> MGSSHHHHHHSQDPMEIDE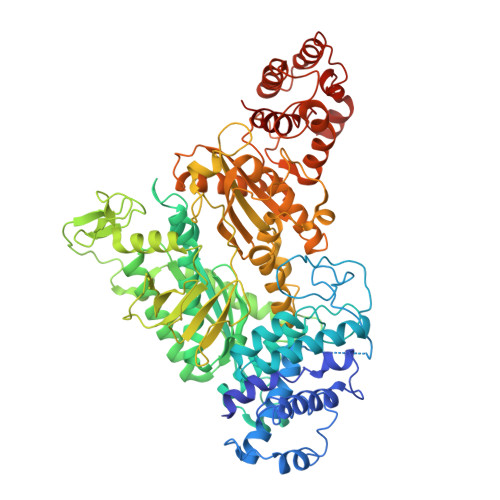LTALGGLLANIGKPVQRAGLYSGDHSTQGARFLRDLAENTGRAEYELLSLFSEFHHKGHMKNDELMIRRIKELSPERFGLTMEDVLNALWIVYEADNLASGEREEGQPQASRPLYSVFNPGKAYPWAELDFEKELPVPGDVFSIRSQDYRELVKRLWEELSKAKLRSDRLLPVLEKYLTFVSSVTSEGNIISLYDHMRMTSAIALAMLRAGCTAEDVRSGRCRKEKRFLLIEGDFSGIQDFIYRVSGKGTLKYLRARSAYLELIGWDVVLEILSRLGLTRANVVFNAGGHFMIIAQNTPDAVKELEEIRAKAVEWLYREFESDLYLAIEWEPVSGREFGREGGKNLFAEARKRLKHKLTVRKLKRFGEIKGLFEHGHTERLAECPVCGRELPEGKLEPSASDPETKVCPTCNRLVSLGGNLPKLLGFGRTAKNDAGVLVEGPFSGFVPYLQGGRPVGEQILVKNTLNPGEIPESAQFVPYFVADYFKKDPKGGVATFEELSMASTGTRRLGVMKGDVDRLGEFFSSMDSPSKLATASRFMDYFFKGYIGAIIEGKFGYIIGDVPSLRDWPEEPDIVVVYAGGDDFFIVGAWDQIFELAFRVRRAFNAYTGGKLTLSVGLGYFDERTPIYRMADVVSERLDTAKDEGRNRVFVVGRSRPLDGKHKLSYEWNHYEELWRTYAPRIYAGNGRLKGKLESKKGLLWKLLEIRELYVRDPNDVRWAYLTAYLLGRHGLSDLFPELVGIDTKAVERKEPQPVYWVDGVLKIVLMAVRR The adaptor protein, speckle-type BTB/POZ protein (SPOP), recruits substrates to the cullin-3-subclass of E3 ligase for selective protein ubiquitylation. SPOP recruits substrates via its N-terminal MATH domain, whereas a central BTB domain mediates dimerization and interactions with Cul3. Here, we show that MyD88 interacts with SPOP through a long degron that contains the established SPOP-binding consensus and an N-terminal site that we name the Q-motif. We determine the structural basis of these interactions and show that the Q-motif interacts with an unexplored binding pocket on the SPOP MATH domain.

We found that the search motif is present in six additional known SPOP substrates – GLI family zinc finger 2 (GLI2), DEK, steroid receptor coactivator-3 (SRC-3; also known as nuclear receptor coactivator 3 (NCoA-3)), sentrin-specific protease 7 (SENP7), SET domain-containing protein 2 (SETD2), and Caprin1. We crystallized SPOPMATH in complex with the 17-mer substrate peptides and obtained high-resolution structures of SPOPMATH in complex with SRC-3, SETD2, and Caprin1. The SRC-3, SETD2, and Caprin1 peptides all interact at the SPOPMATH substrate-binding groove with the same overall backbone conformation as MyD88. In the N-terminal region, the backbone atoms of peptide positions −3,–5, and −6 make identical hydrogen-bond contacts with main chain atoms of SPOP Lys135 and Arg138 and with the side chain of SPOP Tyr83, respectively. At the −4 position, the SRC-3, SETD2, and Caprin1 peptides all contain a glutamine residue corresponding to MyD88 Gln130, and the side chain of this residue makes identical contacts with the backbone carbonyl groups of SPOP Lys115 and Tyr136. The SPOPMATH hydrophobic pocket (SPOP Phe136, Ile137, and Phe141) encompasses the side chains of peptide positions −4 and −5. The SBC regions of the SRC-3, SETD2, and Caprin1 peptides also interact with SPOPMATH as reported in other substrates, with the exception of the SETD2 and SRC-3 residues that deviate from the consensus at the +4 and +5 positions, respectively. Our work also highlights an additional SPOP binding pocket C-terminal of the SBC, as shown by macroH2A and Caprin1 binding. The 17-mer peptides of Caprin1, GLI2, and SRC-3 bound with the highest affinity, whereas the DEK peptides had the lowest-affinity interactions, with little difference between the 17-mer and 9-mer peptides. Similar to MyD88, mutation of the Q-motif abolished the interactions, consistent with the finding that the Q-motif is necessary for interaction of SPOP to these proteins.

>[2x]APKVVKFSYMWTINNFSFCREEMGEVIKSSTFSSGANDKLKWCLRVNPKGLDEESKDYLSLYLLLVSCPKSEVRAKFKFSILNAKGEETKAMESQRAYRFVQGKDWGFKKFIRRDFLLDEANGLLPDDKLTLFCEVSVVQD;>[2x]QPEATQVPLVSSTSEGY ethyl (2~{S},3~{R})-3-(5-bromanylpyridin-2-yl)-2-fluoranyl-3-oxidanyl-propanoate 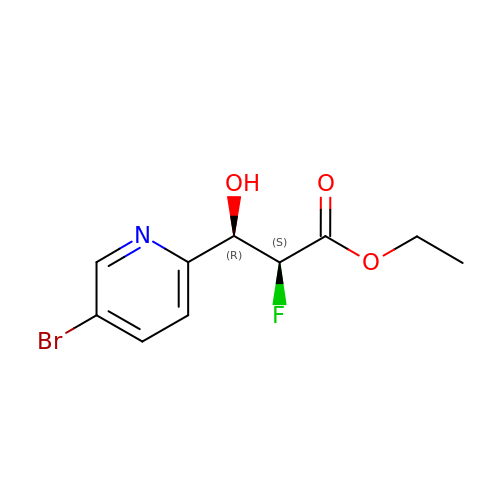| C10 H11 Br F N O3 | JAJULJUIZXJSOC-DTWKUNHWSA-N>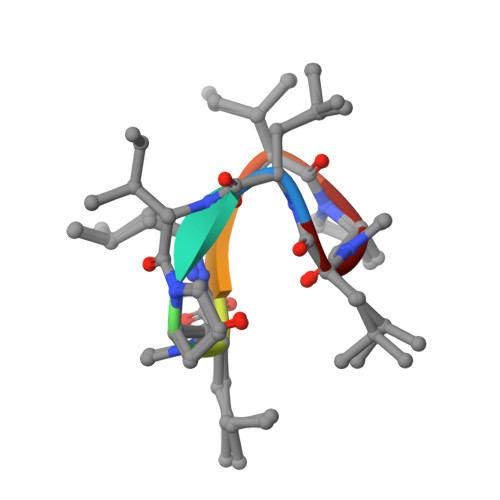 LVPLLIPL The essential and metabolic enzyme adenylate kinase (AK) undergoes large-scale conformational changes in response to binding of its substrates ATP and AMP. In addition to the well-characterized ATP- and AMP-binding domains (ATPlid and AMPbd, respectively), the enzyme has three functional loop segments including the p-loop, the selectivity loop, and the catalytic loop. Here, based on a comparative structure–function analysis of AK enzymes from E. coli and the archaea Odinarchaeota and from human AK1, we found that conformational changes in the enzymes are to a varying degree linked to bending, fraying, or unfolding/folding events of the termini of α-helices observed in various structural hot spots of the enzymes.

In the closed state, however, the side chain of Lys47 shifts rotamer and forms an electrostatic interaction with the side chain of Glu44 located at the N-terminus of the helix. The crystallographic structure of the AKeco Lys47Ala variant in complex with the inhibitor Ap5A was determined to 1.8 Å resolution. As expected, this AKeco variant adopts a structure nearly identical to the native structure and has the ATPlid and AMPbd subdomains in the closed conformation. Structural comparison of the K47-helix in the Lys47Ala variant and in the native Ap5A-bound structure shows that there are no major changes to the helical structure. The observed local helical distortion caused by the side chain of Gln48 binding to the main chain nitrogen atom of Gly45 is further maintained in the Lys47Ala structure. From a functional perspective, the Lys47Ala variant displays a significant increase in k cat relative to the wild type (1.3-fold increase from 360 to 464 s–1), while K M values for the substrates ATP and AMP remain unchanged. The T m of the Lys47Ala variant in apo and Ap5A-bound states decreased with 3.4 and 3.0 °C, respectively, relative to the determined melting points for wild-type AKeco. These differences are significant, and the roughly equal degree of destabilization of the open and closed states indicates that the open-to-closed equilibrium is not affected in the Lys47Ala variant relative to that in the wild type. However, the local destabilization of the K47-helix resulting from the Lys to Ala replacement does correlate with an increased k cat value as observed for the Lys47Ala variant. On the other hand, the Lys47Ala replacement led to a less stable protein with a more dynamic K47-helix and increased catalytic activity.

>[2x]MRIILLGAPGAGKGTQAQFIMEKYGIPQISTGDMLRAAVKSGSELGAQAKDIMDAGKLVTDELVIALVKERIAQEDCRNGFLLDGFPRTIPQADAMKEAGINVDYVLEFDVPDELIVDRIVGRRVHAPSGRVYHVKFNPPKVEGKDDVTGEELTTRKDDQEETVRKRLVEYHQMTAPLIGYYSKEAEAGNTKYAKVDGTKPVAEVRADLEKILG>GPHMGSAAADRRTVEKTWKLMDKVVRLCQNPKLQLKNSPPYILDILPDTYQHLRLILSKYDDNQKLAQLSENEYFKIYIDSLMKKSKRAIRLFKEGKERMYEEQSQDRRNLTKLSLIFSHMLAEIKAIFPNGQFQGDNFRITKADAAEFWRKFFGDKTIVPWKVFRQCLHEVHQISSGLEAMALKSTIDLTCNDYISVFEFDIFTRLFQPWGSILRNWNFLAVTHPGYMAFLTYDEVKARLQKYSTKPGSYIFRLSCTRLGQWAIGYVTGDGNILQTIPHNKPLFQALIDGSREGFYLYPDGRSYNPDLTGLCEPTPHDHIKVTQEQYELYCEMGSTFQLCKICAENDKDVKIEP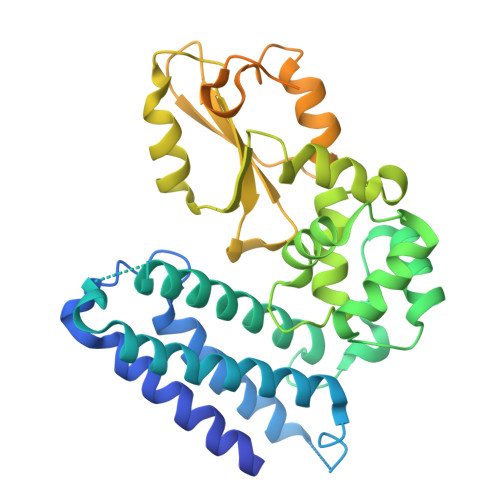CGHLMCTSCLTAWQESDGQGCPFCRCEIKGTEPIIVDPF[3x]>[2x]SMSLPKVMIVVGGQAPKAIRSVECYDFEEDRWDQIAELPSRRCRAGVVFMAGHVYAVGGFNGSLRVRTVDVYDGVKDQ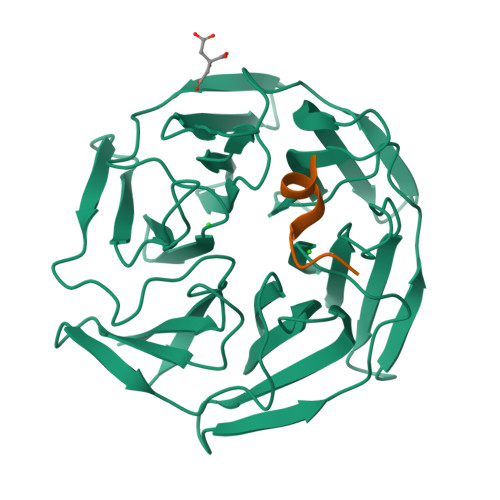WTSIASMQERRSTLGAAVLNDLLYAVGGFDGSTGLASVEAYSYKTNEWFFVAPMNTRRSSVGVGVVEGKLYAVGGYDGASRQCLSTVEQYNPATNEWIYVADMSTRRSGAGVGVLSGQLYATGGHDGPLVRKSVEVYDPGTNTWKQVADMNMCRRNAGVCAVNGLLYVVGGDDGSCNLASVEYYNPVTDKWTLLPTNMSTGRSYAGVAVIHKSL;>ECEETEVDQHV[2x]> FSPTLIADMAKIFMDNYCSPEKLTGMEEAIDAASSNTEILSISDPTMLANVLTDGVKKTISDSRVKVTYEPDLILAAPPAMPDIPLEHLAAMIKGTVKVEILEGNIGYLKIQHIIGEEMAQKVGPLLLEYIWDKILPTSAMILDFRSTVTGELSGIPYIVSYFTDPEPLIHIDSVYDRTADLTIELWSMPTLLGKRYGTSKPLIILTSKDTLGIAEDVAYCLKNLKRATIVGENTAGGTVKMSKM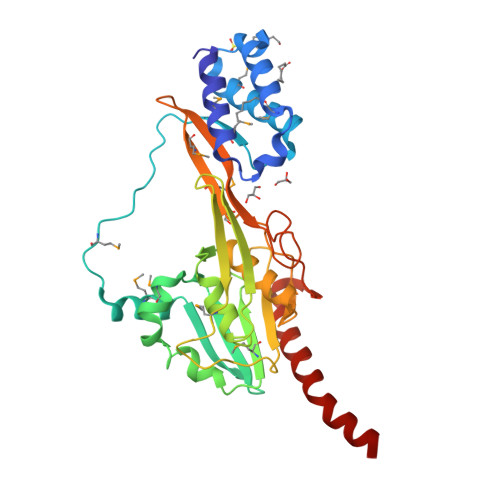KVGDTDFYVTVPVAKSINPITGKSWEINGVAPDVDVAAEDALDAAIAIIKLRAEIPALAQAAAT> MIRMAQNNKELEKLAYEYQVLQAQAQILAQNLELLNLAKAEVQTVRETLENLKKIEEEKPEILVPIGAGSFLKGVIVD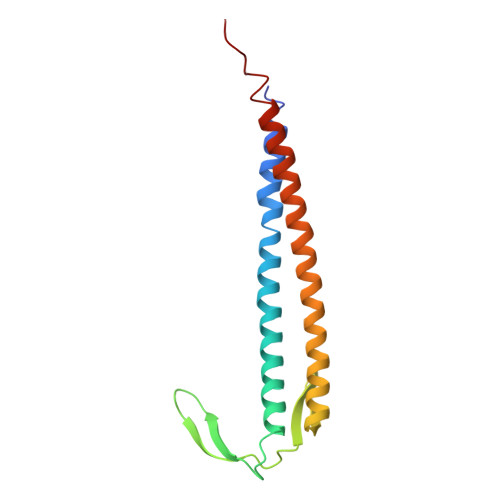KNNAIVSVGSGYAVERSIDEAISFLEKRLKEYDEAIKKTQGALAELEKRIGEVARKAQEVQQKQSMTSFKVKK1-(4-fluorophenyl)thiourea 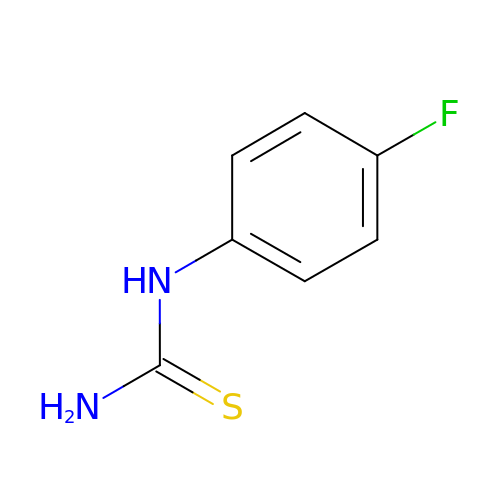| C7 H7 F N2 S | BRWKXKNZRVALNZ-UHFFFAOYSA-N>MAKTKGTASGRGGLGGQGAGGDVIEVGGAGQGGYGGLGSQGTSGRGGLGGQGAGGDVIEVGGAGQGGYGGLGSQGTSGRGGLGGQGAGGDVIEVGGAGQGGYGGLGSQGTSGRGGLG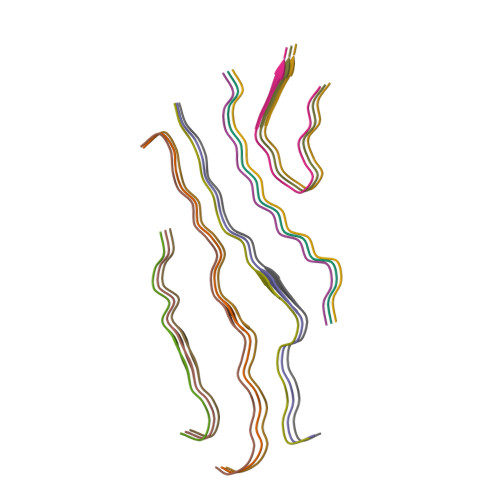GQGAGGDVIEVGGAGQGGYGGLGSQGTSGRGGLGGQGAGGDVIEVGGAGQGGYGGLGSQGTSGRGGLGGQGAGGDVIEVGGAGQGGYGGLGSQGTSGRGGLGGQGAGGDVIEVGGAGQGGYGGLGSQGTSGRGGLGGQGAGGDVIEVGGAGQGGYGGLGSQGTSGRGGLGGQGAGGDVIEVGGAGQGGYGGLGSQGTSGRGGLGGQGAGGDVIEVGGAGQGGYGGLGSQGTSGRGGLGGQGAGGDVIEVGGAGQGGYGGLGSQGTSGRGGLGGQGAGGDVIEVGGAGQGGYGGLGSQGTSGRGGLGGQGAGGDVIEVGGAGQGGYGGLGSQGTSGRGGLGGQGAGGDVIEVGGAGQGGYGGLGSQGTSGRGGLGGQGAGGDVIEVGGAGQGGYGGLGSQGTSGRGGLGGQGAGGDVIEVGGAGQGGYGGLGSQGTSSGHHHHHHHHHH[15x]>MALSTATKAATDALAANRAPTSVNAQEVHRWLQSFNWDFKNNRTKYATKYKMANETKEQFKLIAKEYARMEAVKDERQFGSLQDALTRLNAGVRVHPKWNETMKVVSNFLEVGEYNAIAATGMLWDSAQAAEQKNGYLAQVLDEIRHTHQCAYVNYYFAKNGQDPAGHNDARRTRTIGPLWKGMKRVFSDGFISGDAVECSLNLQLVGEACF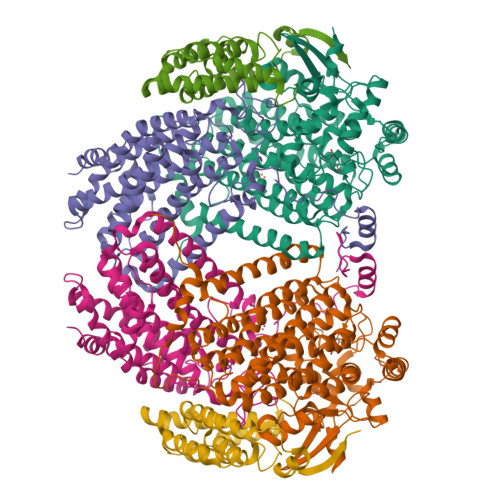TNPLIVAVTEWAAANGDEITPTVFLSIETDELRHMANGYQTVVSIANDPASAKYLNTDLNNAFWTQQKYFTPVLGMLFEYGSKFKVEPWVKTWDRWVYEDWGGIWIGRLGKYGVESPRSLKDAKQDAYWAHHDLYLLAYALWPTGFFRLALPDQEEMEWFEANYPGWYDHYGKIYEEWRARGCEDPSSGFIPLMWFIENNHPIYIDRVSQVPFCPSLAKGASTLRVHEYNGEMHTFSDQWGERMWLAEPERYECQNIFEQYEGRELSEVIAELHGLRSDGKTLIAQPHVRGDKLWTLDDIKRLNCVFKNPVKAFN[2x];>MSMLGERRRGLTDPEMAAVILKALPEAPLDGNNKMGYFVTPRWKRLTEYEALTVYAQPNADWIAGGLDWGDWTQKFHGGRPSWGNETTELRTVDWFKHRDPLRRWHAPYVKDKAEEWRYTDRFLQGYSADGQIRAMNPTWRDEFINRYWGAFLFNEYGLFNAHSQGAREALSDVTRVSLAFWGFDKIDIAQMIQLERGFLAKIVPGFDESTAVPKAEWTNGEVYKSARLAVEGLWQEVFDWNESAFSVHAVYDALFGQFVRREFFQRLAPRFGDNLTPFFINQAQTYFQIAKQGVQDLYYNCLGDDPEFSDYNRTVMRNWTGKWLEPTIAALRDFMGLFAKLPAGTTDKEEITASLYRVVDDWIEDYASRIDFKADRDQIVKAVLAGLK[2x];>[2x]MAKLGIHSNDTRDAWVNKIAQLNTLEKAAEMLKQFRMDHTTPFRNSYELDNDYLWIEAKLEEKVAVLKARAFNEVDFRHKTAFGEDAKSVLDGTVAKMNAAKDKWEAEKIHIGFRQAYKPPIMPVNYFLDGERQLGTRLMELRNLNYYDTPLEELRKQRGVRVVHLQSPH>[6x]GKISTDKYIFLTPRAYIIVHLLKVGKAKASEISENTQIPYQTVIQNIRWL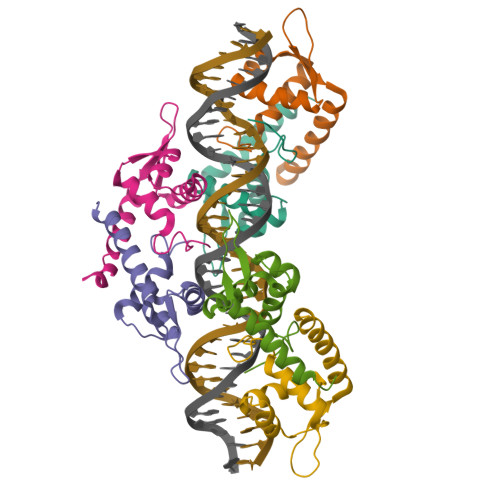LAEGYVVKEQKGEEIYYKLTDKGKQLATAELEKIRKLVEVVQ>GPVDAPILLRQMFEPVSCTFTYLLGDRESREAVLIDPVLETAPRDAQLIKELGLRLLYAVNTHCHADHITGSGLLRSLLPGCQSVISRLSGAQADLHIEDGDSIRFGRFALETRASPGHTPGCVTFVLNDHSMAFTGDALLIRGCGRTDFQQGCAKTLYHSVHEKIFTLP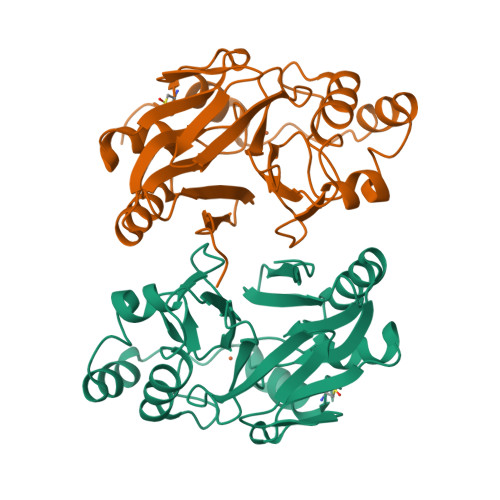GDCLIYPAHDYHGFTVSTVEEERTLNPRLTLSCEEFVKIMGNLNLPKPQQIDFAVPANMRCGVQTPTA[2x]>SNASRDDKKDGVAGPGDAVRVTSSKLVTQPGTSNPKAVVSFYEDFLCPACGIFERGFGPTVSKLVDIGAVAADYTMVAILDSASNQHYSSRAAAAAYCVADESIEAFRRFHAALFSKDIQPAELGKDFPDNARL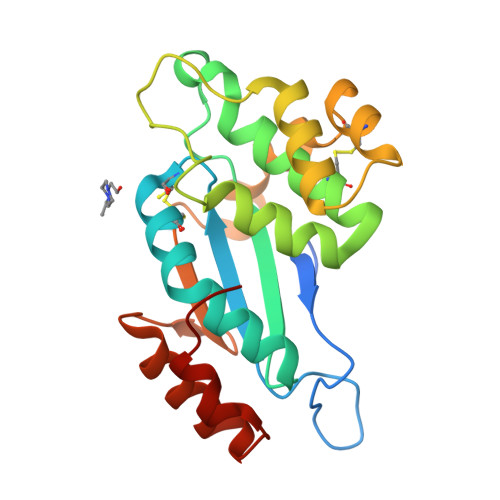IELAREAGVVGKVPDCINSGKYIEKVDGLAAAVNVHATPTVRVNGTEYEWSTPAALVAKIKEIVGDVPGIDSAAATATS[2x]NITs are attractive biocatalysts for the synthesis of amides and carboxylic acids for use in the manufacture of drugs and fine chemicals. We recently discovered that substrate specificity in plant NITs is related to the structure of the NIT helical assembly. The helical twist (Δϕ) of the NIT filament is correlated with the size of the preferred substrate: NIT4 enzymes have a relatively large helical twist, small substrate size, and high specificity, while NIT1 enzymes have a smaller twist and broader specificity. Here we present what we believe to be the first close-to-atomic structure of a full-length active helical NIT (EC 3.5.5.1) using cryo-electron microscopy at a resolution of 3.4 Å.

AtNIT4 is a left-handed helical tube with 4.9 sunbunits (dimers) in one helical turn, a pitch of 8.62 nm, an outer diameter of ~13 nm, and a ~2 nm hollow core. There are two diad axes, which are related to one another by a −5° (negative value: left-handed by convention) rotation and 4.31 nm translation along the helical axis. The extended C-terminal tail of each monomer forms two ß-strands, which assemble, along with strands from monomers across the A- and C-interfaces, into a row of 4-stranded ß-sheets in the interior of the tubular filament. Interactions across the helical groove (D- or F-interfaces) were not observed and this could explain the plasticity of NIT helical twist. AtNIT4 shows high-structural homology with other members of the NIT superfamily including a conserved αßßα core and CEEK catalytic tetrad. The substrate-binding pocket is a ~7 × 4 Å tunnel lying close to the C-interface that runs almost perpendicular to the helical axis. The NIT superfamily binding pocket has been described, but in addition to these shared elements, in AtNIT4 a loop from the adjacent monomer extends over the C-interface in line with C197. Crucially, we observed via molecular dynamics, that this loop is held in position by a charge–charge interaction between R95 and D317. On this basis we refer to the loop as a lid, R95 as a lock, and the flexible ends of the loop as a hinge, which open or close, shifting the lid relative to C197. We propose: R95T eliminates the positive charge at position 95, which disrupts the interaction with D317 and allows the lid loop to open and shift away from C197.

>[12x]MSMQQETSHMTAAPQTNGHQIFPEIDMSAGDSSSIVRATVVQASTVFYDTPATLDKAERLLSEAAENGSQLVVFPEAFIGGYPRGSTFELAIGSRTAKGRDDFRKYHASAIDVPGPEVERLALMAKKYKVYLVMGVIEREGYTLYCTVLFFDSQGLFLGKHRKLMPTALERCIWGFGDGSTIPVFDTPIGKIGAAICWENRMPSLRTAMYAKGIEIYCAPTADSRETWLASMTHIALEGGCFVLSANQFCRRKDYPSPPEYMFSGSEESLTPDSVVCAGGSSIISPLGIVLAGPNYRGEALITADLDLGDIARAKFDFDVVGHYSRPEVFSLNIREHPRKAVSFKTSKVMEDESVHHHHHH>HHHHHHMSAKDERAREILRGFKLNWMNLRDAETGKILWQGTEDLSVPGVEHEARVPKKILKCK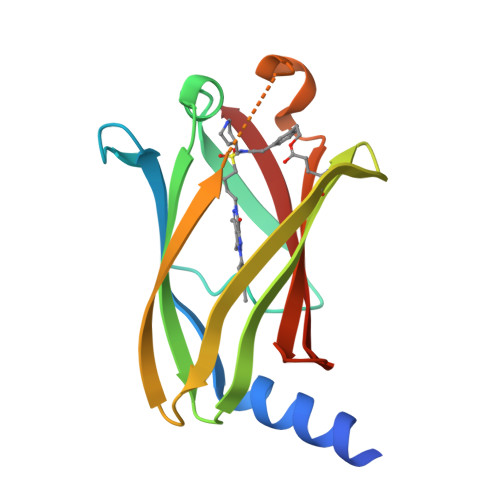AVSRELNFSSTEQMEKFRLEQKVYFKGQCLEEWFFEFGFVIPNSTNTWQSLIEAAPESQMMPASVLTGNVIIETKFFDDDLLVSTSRVRLFYV[2x]> MISDEQLNSLAITFGIVMMTLIV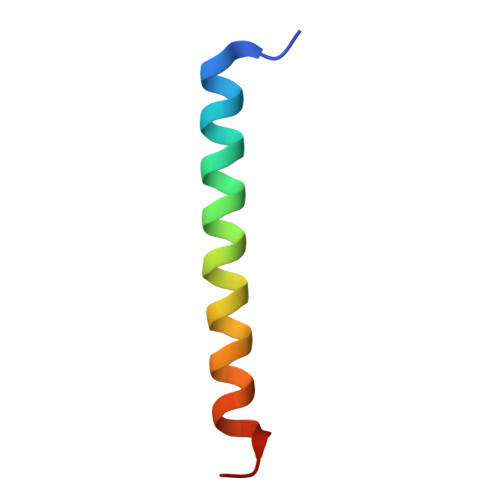IYHAVDSTMSPKN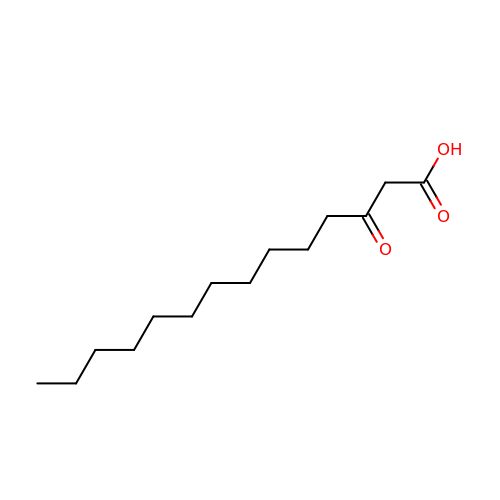3-oxotetradecanoic acid | C14 H26 O3 | XLKOZYOVXNPWGT-UHFFFAOYSA-N> MGSSHHHHHHSSGRENLYFQGMRVLVVGANGKVARYLLSELKNKGHEPVAMVRNEEQGPELRERGASDIVVANLEEDFSHAFASIDAVVFAAGSGPHTGADKTILIDLWGAIKTIQEAEKRGIKRFIMVSSVGTVDPDQGPMNMRHYLVAKRLADDELKRSSLDYTIVRPGPLSNEESTGKVTVSPHFSEITRSITRHD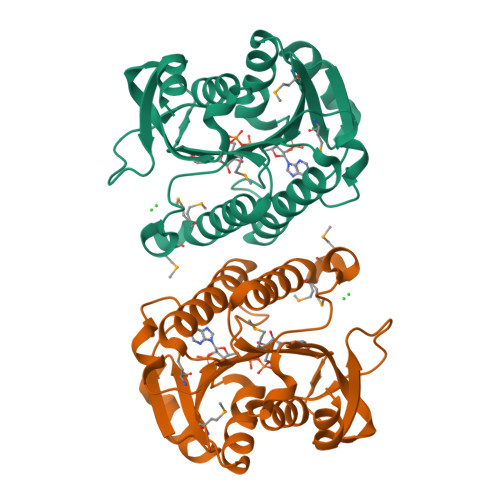VAKVIAELVDQQHTIGKTFEVLNGDTPIAKVVEQLGS In eukaryotes, HDACs, which belong to the epigenetic machinery of the cells, catalyze the deacetylation of ϵ‐amino groups of lysine residues in histone tails, leading in consequence to a more compact chromatin structure, which usually results in an inhibition of transcription. In contrast to hsHDAC8, showing in humans the lowest level of expression of the class I enzymes, in S. mansoni smHDAC8 is the most abundantly expressed class I HDAC at all life‐cycle stages and was validated as drug target for schistosome‐specific inhibitors. The active sites of the enzymes consist of a long narrow tunnel, accommodating the incoming acetylated lysine side chain of the substrate, which leads to a cavity containing the catalytic Zn2+‐ion. The active site residues of the two enzymes are highly conserved, with only M274 in hsHDAC8, being substituted by H292 in smHDAC8.6 The replacement of this hydrophobic residue by a polar one modifies the physicochemical properties of the active site, which could be exploited for the development of smHDAC8‐specific inhibitors.

In this study, initial screening revealed the triazole‐based hydroxamate 2 b (N‐hydroxy‐1‐phenyl‐1H‐1,2,3‐triazole‐4‐carboxamide) exhibiting potent inhibitory activity toward the novel antiparasitic target Schistosoma mansoni histone deacetylase 8 (smHDAC8) and promising selectivity over the major human HDACs. Due to the promising biological activity of the 1‐phenyl substituted triazole derivative 2 b, the compound was crystallized in complex with smHDAC8. The structure reveals that compound 2 b binds in the smHDAC8 active site in a straight conformation, its capping group pointing toward the solvent, whereas its hydroxamate moiety forms a bidentate interaction with the catalytic zinc ion as well as hydrogen bonds with the side chains of histidines H141 and H142 and the hydroxyl group of catalytic tyrosine Y341. Interestingly, the triazole ring of 2 b is observed almost stacked between the side chains of phenylalanines F151 and F216 that form the active site tunnel normally accommodating the aliphatic part of the incoming acetylated lysine side chain. Yet, the F151 side chain is observed in two conformations, one turned toward the active site, participating to the tunnel mentioned previously, and one turned away from the active site. This suggests that the stacking of the triazole ring between the two phenylalanines observed in the structure is not absolutely essential for the interaction. In addition, the nitrogen atoms of the triazole ring are not facing the smHDAC8‐specific H292 side chain but turned toward the Cα carbon atom of glycine G150. Finally, the capping group of 2 b does not appear to make extensive interactions with smHDAC8. Yet, the rather small size of the inhibitor allows it to fit nicely into the smHDAC8 active site pocket. Replacement of smHDAC8 H292 by the somewhat bulkier human methionine M274 could potentially explain the increased IC50 for 2 b measured with the human enzyme.

>[4x]HMSVGIVYGDQYRQLCCSSPKFGDRYALVMDLINAYKLIPELSRVPPLQWDSPSRMYEAVTAFHSTEYVDALKKLQMLHCEEKELTADDELLMDSFSLNYDCPGFPSVFDYSLAAVQGSLAAASALICRHCEVVINWGGGWHHAKRSEASGFCYLNDIVLAIHRLVSSTPPETSPNRQTRVLYVDLDLHHGDGVEEAFWYSPRVVTFSVHHASPGFFPGTGTWNMVDNDKLPIFLNGAGRGRFSAFNLPLEEGINDLDWSNAIGPILDSLNIVIQPSYVVVQCGADCLATDPHRIFRLTNFYPNLNLDSDCDSECSLSGYLYAIKKILSWKVPTLILGGGGYNFPDTARLWTRVTALTIEEVKGKKMTISPEIPEHSYFSRYGPDFELDIDYFPHESHNKTLDSIQKHHRRILEQLRNYADLNKLIYDYDQVYQLYNLTGMGSLVPR> MEKLVQPTPLLLSLLKSAGAQKETFTMKEVLYHLGQYIMA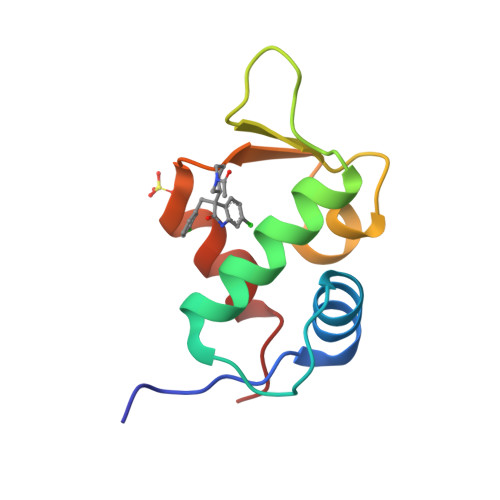KQLYDEKQQHIVHCSNDPLGELFGVQEFSVKEHRRIYAMISRNLVS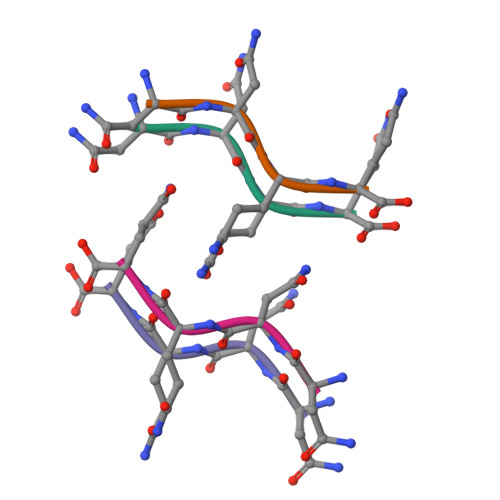> NNQQ>MSQVTDMRSNSQGLSLTDSVYERLLSERIIFLGSEVNDEIANRLCAQILLLAAEDASKDISLYINSPGGSISAGMAIYDTMVLAPCDIATYAMGMAASMGEFLLAAGTKGKRYALPHARILMHQPLGGVTGSAADIAIQAEQFAVIKKEMFRLNAEFTGQPIERIEADS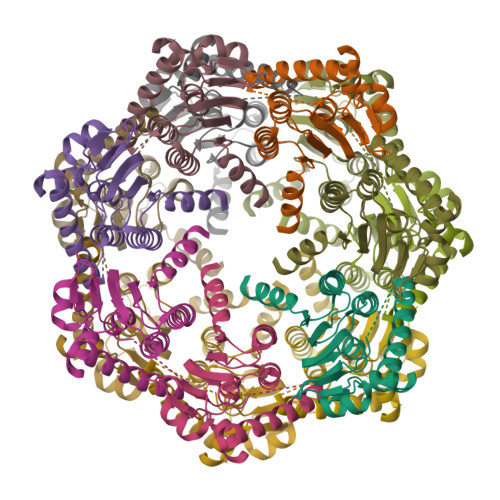DRDRWFTAAEALEYGFVDHIITRAHVNGEAQ[14x]> MKILLIGMGGTIASVKGENGYEASLSVKEVLDIAGIKDC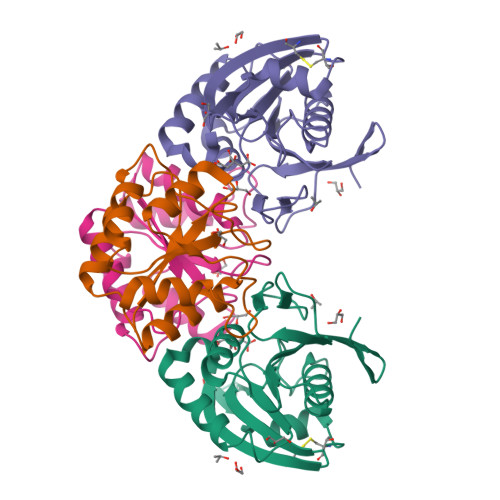EDCDFLDLKNVDSTLIQPEDWVDLAETLYKNVKKYDGIIVTHGTDTLAYTSSMISFMLRNPPIPIVFTGSMIPATEENSDAPLNLQTAIKFATSGIRGVYVAFNGKVMLGVRTSKVRTMSRDAFESINYPIIAELRGEDLVVN;> MAVLVIKLIPGLSGDIFRAAVELGYRGIVIEGYGAGGIPYRGSDLLQTIEELSKEIPIVMTTQAMYDGVDLTRYKVGRLALRAGVIPAGDMTKEATVTKLMWILGHTNNVEEIKVLMRKNLVGELRD6-phenyl-N-(pyridin-4-yl)pyrrolo[2,1-f][1,2,4]triazin-4-amine 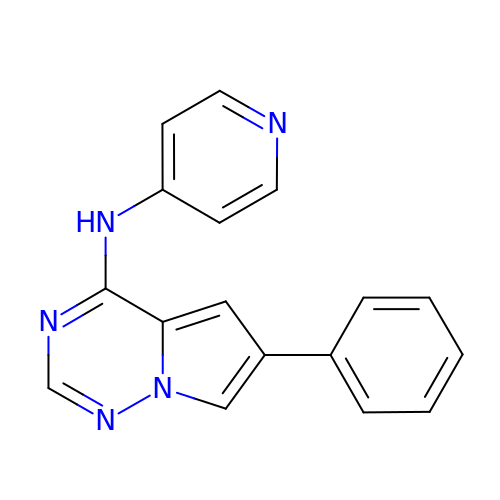| C17 H13 N5 | KOECVTWSFPGZJE-UHFFFAOYSA-N>MSNAVLYKSNHNVVYSCKYHIVWCPKYRRKVLVGAV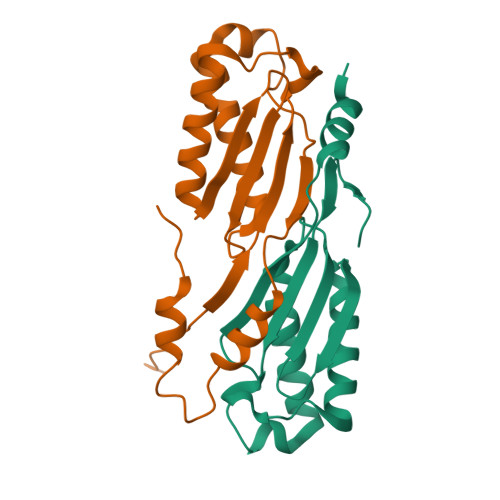EMRLKEIIQEVAKELRVEIIEMQTDKDHIHILADIDPSFGVMKFIKTAKGRSSRILRQEFNHLKTKLPTLWTNSCFISTVGGAPLNVVKQYIENQQNSNRPKQKEKWKSYVDNLQTKAL[2x]> KAVITLQP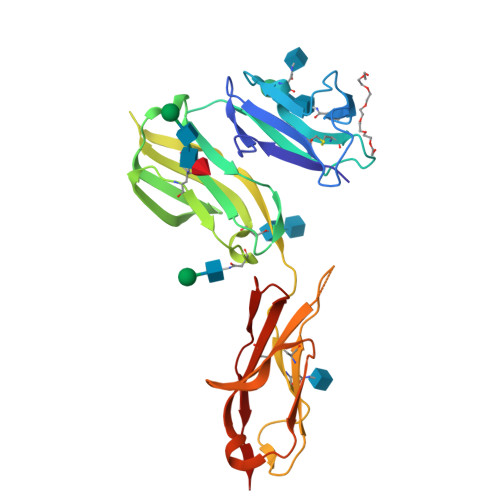PWVSVFQEETVTLHCEVLHLPGSSSTQWFLNGTATQTSTPSYRITSASVNDSGEYRCQRGLSGRSDPIQLEIHRGWLLLQVSSRVFTEGEPLALRCHAWKDKLVYNVLYYRNGKAFKFFHWNSNLTILKTNISHNGTYHCSGMGKHRYTSAGISVTVKELFPAPVLNASVTSPLLEGNLVTLSCETKLLLQRPGLQLYFSFYMGSKTLRGRNTSSEYQILTARREDSGLYWCEAATEDGNVLKRSPELELQVLG>MGHHHHHHMPEINTNHLDKQQVQLLAEMCILIDENDNKIGAETKKNCHLNENIEKGLLHRAFSVFLFNTENKLLLQQRSDAKITFPGCFTNTCCSHPLSNPAELEESDALGVRRAAQRRLKAELGIPLEEVPPEEINYLTRIHYKAQSDGIWGEHEIDYILLVRMNVTLN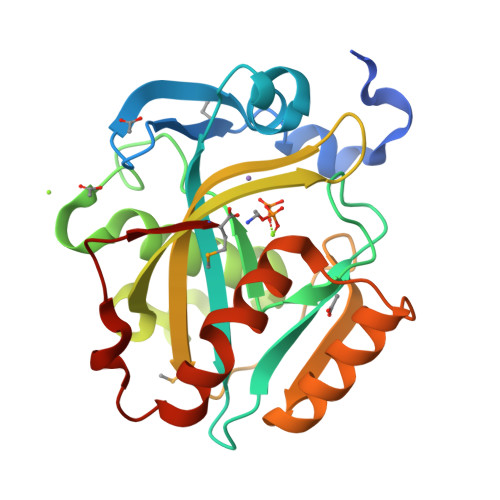PDPNEIKSYCYVSKEELKELLKKAASGEIKITPWFKIIAATFLFKWWDNLNHLNQFVDHEKIYRM[2x]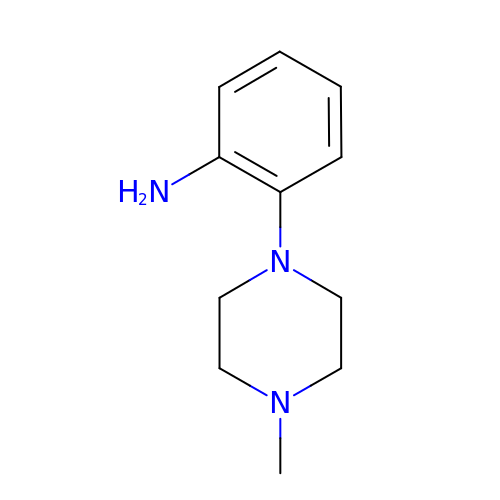2-(4-methylpiperazin-1-yl)aniline | C11 H17 N3 | INWHDRNGZMHXEZ-UHFFFAOYSA-N Coxsackie B viruses (CVBs) belong to the Enterovirus (EV) B species of the Picornaviridae family and are divided into six serotypes (CVB1-CVB6). The structural proteins VP1-VP4 form protomers, and five of these protomers assemble into a pentamer. Finally, an icosahedral capsid, approximately 30 nm in diameter, consists of 12 pentamers. VP1, VP2, and VP3 are exposed on the particle surface, whereas VP4 is an internal protein.

The immunodominant PALXAXETG motif, located in the VP1 N-terminus, is a highly conserved region in enteroviruses that elicits non-neutralizing antibody responses. On the basis of studies reporting the most immunoreactive parts of the PALXAXETG motif, we excluded the 15 amino acid-long region SESIPALTAAETGHT from the VP1 N-terminus of CVB1 and designated the deletion PALXA. Using this modified construct, we produced a VLP denoted VLPΔpalxa. SDS‒PAGE and total protein staining of the capsid proteins confirmed the presence of proteins of approximately 38 kDa, 29.5 kDa and 26 kDa corresponding to the expected molecular sizes of VP0, VP1 devoid of 15 amino acids from the N-terminus, and VP3, respectively. The results of the quality analyses and structural determination revealed that the 15 amino acid deletion from VLPΔpalxa did not prevent particle formation. The melting temperature (Tm) of VLPΔpalxa was 69.05 °C ± 0.05, which is comparable to that of unmodified VLP (Tm 69.78 °C ± 0.09), indicating that the modification did not compromise the thermostability of the particles. Notably, the yield of VLPΔpalxa was 29.5 mg/l, which was 2.5 times higher than the yield of the previously produced unmodified VLP, indicating that the particle stability may have increased compared with that of the unmodified VLP. We successfully engineered CVB1-VLPs lacking the conserved PALXAXETG motif without compromising particle formation or structural integrity, as confirmed by high-resolution structural analysis. As expected, the VLPΔpalxa-vaccinated group was negative for antibodies recognizing this epitope, whereas only the formalin-inactivated virus group elicited a significant response toward this peptide, with a GMT of 1089 (p = 0.004). To summarize, we demonstrated that targeted structural modification of the CVB1-VLP capsid can reduce immunodominant antibody responses, especially those directed against the conserved PALXAXETG motif after vaccination.

>[20x]GPVEESVERAMVRVADTVSSRPTNSQVVPSDTMQTRHVKNYHSRSESSIENFLCRAACVYYATYTNNSEKGYAEWVINTRQVAQLRRKLELFTYLRFDLELTFVITSAQQPSTATSVDAPVQTHQIMYVPPGGPVPTKVTDYAWQTSTNPSVFWTEGNAPPRMSIPFISIGNAYSCFYDGWTQFSRNGVYGINTLNNMGTLYMRHVNEAGQGPIKSTVRIYFKPKHVKAWVPRPPRLCQYEKQKNVNFTPTGVTTTRVGITTT;>SPSAEECGFSDRVRSITLGNSTITTQECANVVVGYGVWPEYLKDNEATAEDQPTQPDVATCRFYTLESVQWMKNSAGWWWKLPDALSQMGLFGQNMQYHYLGRTGYTIHVQCNASKFHQGCLLVVCVPEAEMGCSNLNNTPEFAELSGGDTARMFTDTQIGETNSKKVQTAVWNAGMGVGVGNLTIYPHQWINLRTNNSATIVMPYINSVPMDNMFRHNNLTLMIIPFVPLNYSEGSSPYVPITVTIAPMCAEYNGLRLASSQ[20x];>GLPVMTTPGSTQFLTSDDFQSPSAMPQFDVTPEMQIPGRVNNLMEIAEVDSVVPVNNTEANVNSLKAYQIPVQSNSDNGKQVFGFPLQPGANGVLNRTLLGEILNYYTHWSGSIKLTFMFCGSAMATGKFLLAYSPPGAGVPKNRKDAMLGTHVIWDVGLQSSCVLCVPWISQTHYRYVVEDEYTAAGYITCWYQTNIVVPADVQSSCDILCFVSACNDFSVRMLKDTPFIRQDTFYQ[20x];>[10x]MGAQVSTQKTGAHETGLNASGNSIIHYTNINYYKDAASNSANRQDFTQDPGKFTEPVKDIMIKSMPALN>MALLTPIPSPMVNLTQVIDPTEQLAYFPKITFERLKNYDTSSNYAKGKLTRNYMILLPWQHVNRYNFVFSSTGCKVSLKTCIGKLMKDLNPKVLYFIGEGAGNWMARTACEYPDIKFVYRSLKDDLDHHYPLEYQRVIGELSRIIDSGEGLSMETTDATQKTHWDLIHRVSKDALLITLCDAEFKDRDDFFKMVILWRKHVLSCRICTTYGTDLYLFAKYHAKDCNVKLPFFVRSVATFIMQGSKLSGSECYILLTLGHHNNLPCHGEIQNSKMKIAVCNDFYAAKKLDNKSIEANCKSLLSGLRIPINKKELNRQRRLLTLQSNHSSVATVGGSKVIE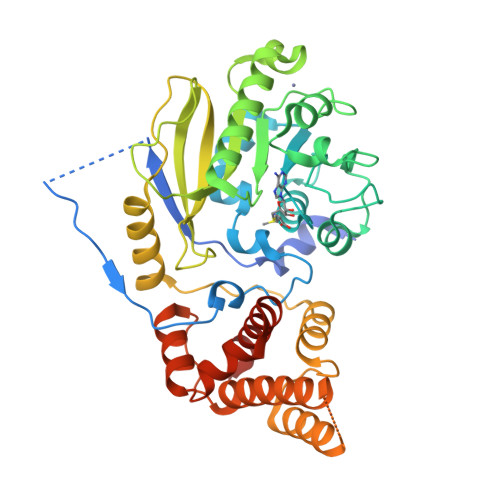SKWLTNKANTIIDWLEHILNSPKGELNYDFFEALENTYPNMIKLIDNLGNAEIKKLIEVTGYMLVSKKSGHHHHHH[2x]>[2x]VTAYEEIVCQVFAAVLDRSDVTADADFFALGGHSLLSLRVVARLRALLGVDVGVRDLFEAPTPAALAARLTTQTGRRPAVTRRGPDAPPVLSHFQRRLWLIEQVYQTRGAYNVPLAVHVSDRLDLDVLRAAVRDLVARHEVLRTLVRSSDDGPDPVLLAPED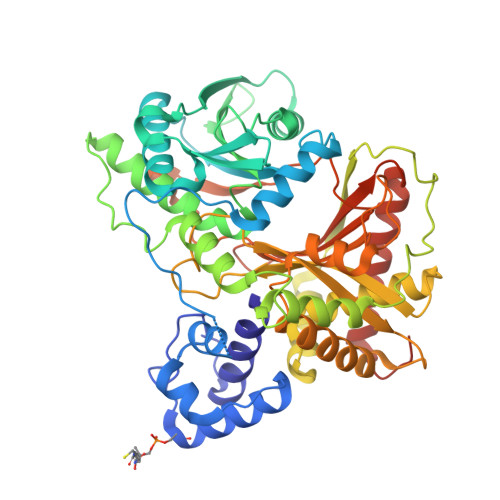AAVDVAEVQAAGPVADLLAELTAQPFDLATQIPLRVRMITGEQVDGCVLLLVCHHIAADEWSFAPLLRDLDTAYRARAAGRAPDWEPLPAQYSDYAATLHDWLGEATDPASPLRRQLDYWQHALQDLPDELDLPTDRPRPATASHRGGLARAELPPELVEAVRRLAAQHGVTVFMVVQAAVAVLLHRLGAGDDIPLGSPVADRADEAVHDTVGFFLNTLVLRVNLSGNPTFADLLDRVRAVDLEAFARADAPFDAVVDTVKPPRAVSRHPLFQTMVSYQRRPSDVDRLFGAATRLVEVPLDTAKFDLEFAFIEDGHGGAHIALNYAADLFDHDSAEQLVARLRTVLEHACADPCRPVAGVEVVSGA>SGFYHKHFLKLLDFTPAELNSLLQLAAKLKADKKSGKEEAKLTGKNIALIFEKDSTRTRCSFEVAAYDQGARVTYLGPSGSQIGHKESIKDTARVLGRMYDGIQYRGYGQEIVETLAEYARVPVWNGLTNEFHPTQLLADL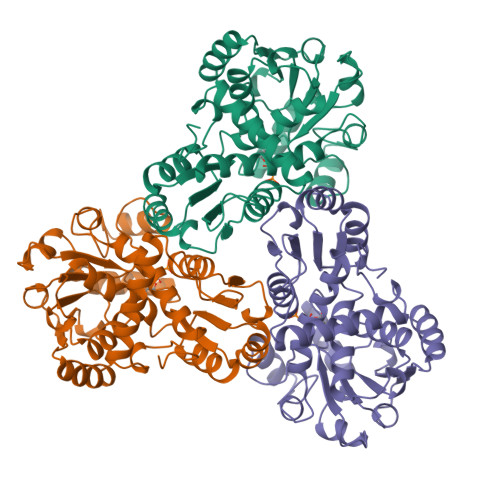LTMQEHLPGKAFNEMTLVYAGDARNNMGNSMLEAAALTGLDLRLVAPQACWPEAALVTECRALAQQNGGNITLTEDVAKGVEGADFIYTDVWVSMGEAKEKWAERIALLREYQVNSKMMQLTGNPEVKFLHCLPAFHDDQTTLGKKMAEEFGLHGGMEVTDEVFESAASIVFDQAENRMHTIKAVMVATLSK[9x]> MTNFDKISKMFWHYKDKIAQIKQDIVLPIKKADVNVRNLLSRHKRKINPKFGQLTNSNQQLFKIQNELTQLINDTKGDSLAYHWILNFIAKAVVHQAETEVRVKPESALPLGKLTLYLLVQFPELQELFMARLVKKCPFVIGFTCEIDTEKGRQNMGWKRNNENKWEDNTSYDERMGGILSLFAIITRLQLPQEFITTTSHPFPIALSWHILARICNTPLNLITNTHFVILGSWWDAAAVQFLQAYGNQASKLLILIGEELTSRMAEKKYVGA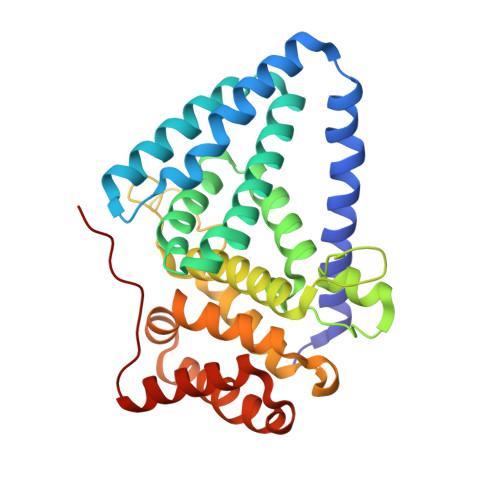ARLRILLEAWQNNNMESFPEMSP>[2x]SMKQTGYLTIGGQRYQAEINDLENLGEMGSGTCGQVWKMRFRKTGHVIAVKQMRRSGNKEENK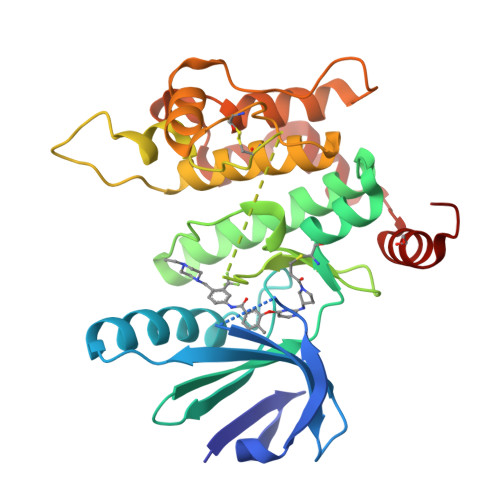RILMDLDVVLKSHDCPYIVQCFGTFITNTDVFIAMELMGTCAEKLKKRMQGPIPERILGKMTVAIVKALYYLKEKHGVIHRDVKPSNILLDERGQIKLCDFGISGRLVDDKAKDRSAGCAAYMAPERIDPPDPTKPDYDIRADVWSLGISLVELATGQFPYKNCKTDFEVLTKVLQEEPPLLPGHMGFSGDFQSFVKDCLTKDHRKRPKYNKLLEHSFIKRYETLEVDVASWFKDVMAKTESPR Saccharomyces cerevisiae possesses two predicted CHI-like proteins, Aim18p (encoded by YHR198C) and Aim46p (YHR199C), but it lacks other enzymes of the flavonoid pathway, suggesting that Aim18p and Aim46p employ the CHI fold for distinct purposes. Here, we demonstrate using proteinase K protection assays, sodium carbonate extractions, and crystallography that Aim18p and Aim46p reside on the mitochondrial inner membrane and adopt CHI folds, but they lack select active site residues and possess an extra fungal-specific loop. Consistent with these differences, Aim18p and Aim46p lack CHI activity and also the fatty acid–binding capabilities of other CHI-like proteins, but instead bind heme. We further show that diverse fungal homologs also bind heme and that Aim18p and Aim46p possess structural homology to a bacterial hemoprotein.

Full-length constructs of Aim18p and Aim46p possessing N-terminal 8X-His tags were insoluble, but truncating the N-terminal mitochondrial targeting sequence and transmembrane domain for Aim18p and Aim46p (Aim18p-Nd70 and Aim46p-Nd62, respectively) dramatically increased solubility. We also generated point mutations of the CHI catalytic arginine—Aim18p-Nd70-R123A and Aim46p-Nd62-R107A—to serve as experimental controls. Each protein exhibited robust thermal melt temperatures ranging from ∼48 to 67 °C, indicating stably folded protein. Interestingly, catalytic arginine mutants lacked this golden color. We used a fluorescent heme detection assay that uses heated oxalic acid to liberate the heme molecule of its central iron metal, generating a fluorescent protoporphyrin molecule. This experiment revealed that Aim18p and Aim46p coimmunoprecipitated with bound heme and that mutating the catalytic arginine significantly reduced heme binding. Alignments of the Aim18-Nd70-R123A and Aim46-Nd62-WT structures with the bacterial protein revealed that, while the α-helices differed substantially, the core CHI antiparallel β-sheet was structurally homologous to the core antiparallel β-sheet of cytochrome c'β-Met. Of note is a region of the Aim18p-Nd70 and Aim46-Nd62 structures that lies in between plant CHI α1 and α2. This region contains an extra loop that is absent in plant CHI domain–containing proteins but is conserved across multiple ascomycete Aim18p and Aim46p homologs. Nearly all of the CHI catalytic residues are substituted nonconservatively in Aim18p and Aim46p except for the catalytic arginine, which is invariably conserved in fungal homologs of Aim18p and Aim46p. Although our data show that the conserved CHI arginine does influence heme binding in Aim18p and Aim46p, it is most likely not the only heme-coordinating residue; future experiments will be necessary to fully understand the coordination environment between heme and the CHI domain.

> RPVQNDDKTDAFPSHTESIQVDSSVSDFPLTITALNFPVSTTFKLLGYGQAHVTFLRFKVYALGLYLAENDENLVSDTLNETYLHKYFLDVDDSKTPKENLARLLKRDDSKSVMMIDDLLDSGMRMLAKITPVRNTDFKHLKEGLVKTISKHPDVANNKDTLAKGLSELNDAFSRKGSVRKNDDLIIELLANGALQFSYHDSKNNEFEVMGVVNNQLVGKFLFSQYLCGEKSPSPQAKKTAIDKLITLL> MKIKPVKVESIENPKRFLNSRLLTKIEVEEAIEKALKQLYINIDYFGEEYPTPATFNNIYKVMDNTEWTNGFWTGCLWLAYEYNQDKKLKNIAHKNVLSFLNRINNRIALDHHDLGFLYTPSCTAEYRINGDVKALEATIKAADKLMERYQEKGGFIQAWGELGYKEHYRLIIDCLLNIQLLFFAYEQTGDEKYRQVAVNHFYASANNVVRDDSSAFHTFYFDPETGEPLKGVTRQGYSDESSWARGQAWGIYGIPLSYRKMKDYQQIILFKGMTNYFLNRLPEDKVSYWDLIFTDGSGQPRDTSATATAVCGI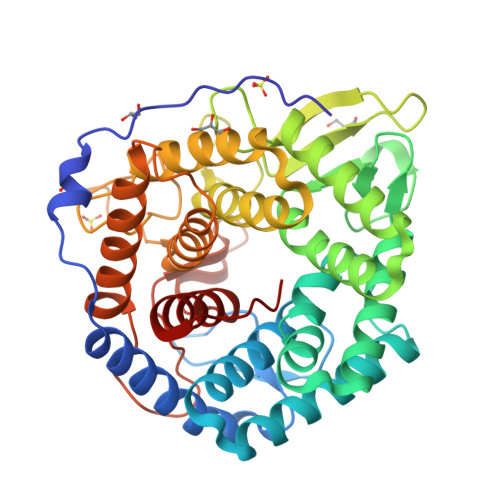HEMLKYLPEVDPDKETYKYAMHTMLRSLIEQYSNNELIAGRPLLLHGVYSWHSGKGVDEGNIWGDYYYLEALIRFYKDWELYW1-(1,4-dimethyl-1,2,3,4-tetrahydroquinoxalin-6-yl)methanamine 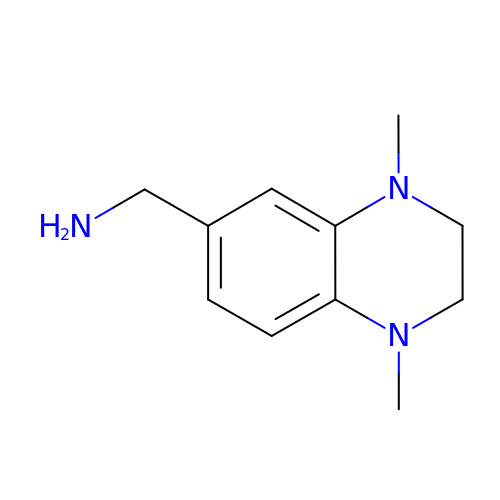| C11 H17 N3 | TWGYATHIWDUKGY-UHFFFAOYSA-N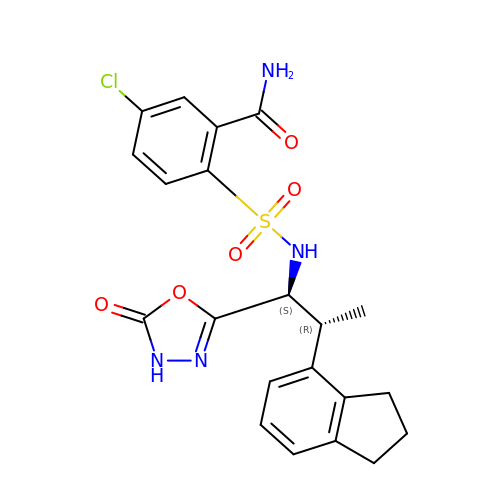5-chloro-2-(N-((1S,2R)-2-(2,3-dihydro-1H-inden-4-yl)-1-(5-oxo-4,5-dihydro-1,3,4-oxadiazol-2-yl)propyl)sulfamoyl)benzamide | C21 H21 Cl N4 O5 S | QYEZTBVHXSYEIR-ZMZPIMSZSA-N> EVANPEHYIKHPLQNRWALWFF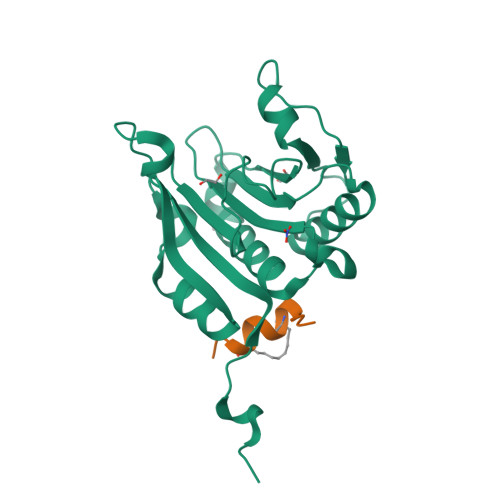KNDKSKTWQANLRLISKFDTVEDFWALYNHIQLSSNLMPGCDYSLFKDGIEPMWEDEKNKRGGRWLITLNKQQRRSDLDRFWLETLLCLIGESFDDYSDDVCGAVVNVRAKGDKIAIWTTECENREAVTHIGRVYKERLGLPPKIVIGYQSHADTATKSGSTTKNRFVV;> XKKRYSRLQLLLFRRR> MANRSRTEAESWYQTKYEELQQTAGRHGDDLRNTKHEISEMNRMIQRLRAEIDNVKKQCANLQNAIADAEQRGELALKDARNKLAELEEALQKAKQDMARLLREYQE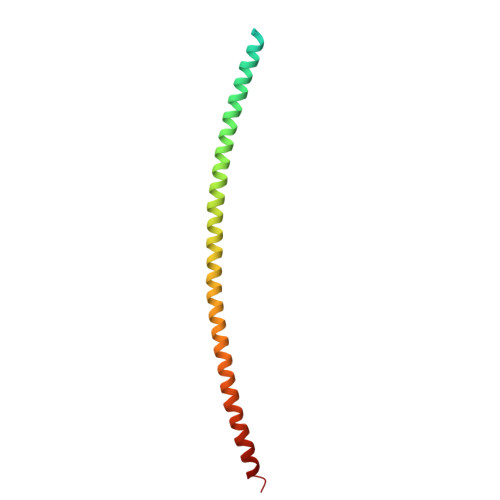LMNTKLALDVEIATYRKLLEGE The DNA damage response protein 53BP1 (p53-binding protein 1) influences the cell cycle dependency of DNA double-strand break (DSB) repair pathway selection. The localization of 53BP1 to chromatin also requires that it binds histone H4 di-methylated at K20 (H4K20me2) via a tandem Tudor domain (53BP1TT), while BRCA1-BARD1 recruitment requires unmethylated H4K20 recognized by an Ankyrin repeat domain in BARD1. We show that a series of water-soluble small molecules targeting the methyl-lysine binding cavity in 53BP1TT function by stabilizing a previously unknown lowly populated autoinhibited homodimeric state of 53BP1TT in which the histone binding surface of H4K20me2 is buried within the protomeric interface. Our work therefore identifies an auto-associated form of 53BP1—autoinhibited for chromatin binding—that can be stabilized by small molecule ligands encapsulated between two 53BP1 protomers.

A low resolution (3.79 Å) model of 53BP1TT-CC derived from X-ray crystallography data was sufficient to demonstrate that both protomers were arranged similarly as wild-type 53BP1TT bound to our small molecules with a root-mean-square deviation for backbone atoms of 0.94 Å. Using NMR spectroscopy, we independently verified that 53BP1TT-CC mimicked the homodimeric state of 53BP1TT bound to UNC3474. Noticeably, the addition of UNC3474 led to the splitting of several NMR signals in the 1H-15N HSQC spectra of 53BP1TT-CC. The addition of the reducing agent dithiothreitol (DTT) changed 53BP1TT-CC to a monomeric state as expected, which, like 53BP1TT-PN, had no affinity for UNC3474. We therefore created 53BP1TT variants that can be switched on and off in vitro for ligand binding. As we showed in vitro, 53BP1TT-PN and reduced-state 53BP1TT-CC cannot dimerize and are thus insensitive to UNC3474 and to the related, lower affinity compounds UNC2170 and UNC2991.

>[10x]GPGHMNSFVGLRVVAKWSSNGYFYSGKITRDVGAGKYKLLFDDGYECDVLGKDILLCDPIPLDTEVTALSCDEYFSAGVVKGHRKESGCLYYSIEKEGQRKWYKRMAVILSLEQGNRLREQYGLG> AYVINEACISCGACE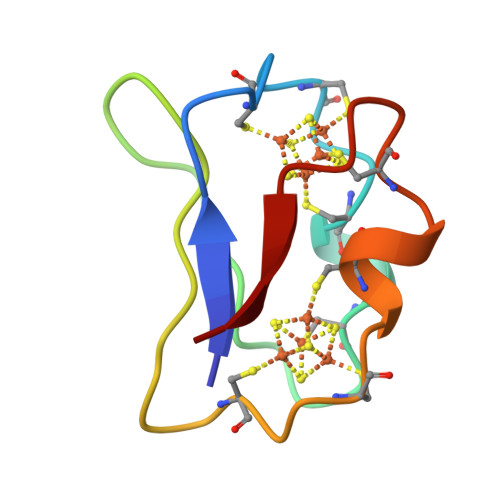PECPVDAISQGGSRYVIDADTCIDCGACAGVCPVDAPVQA> ASDR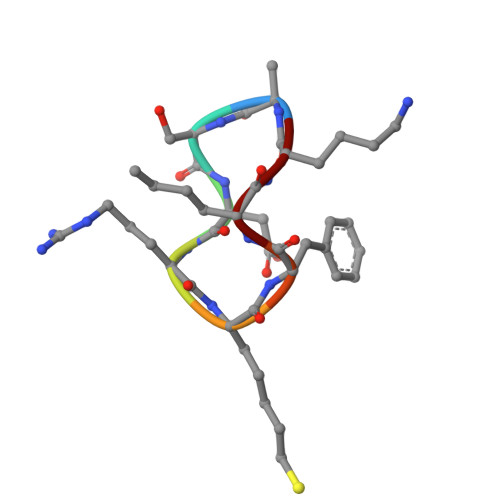XFLK> MALMTWTAAEFGT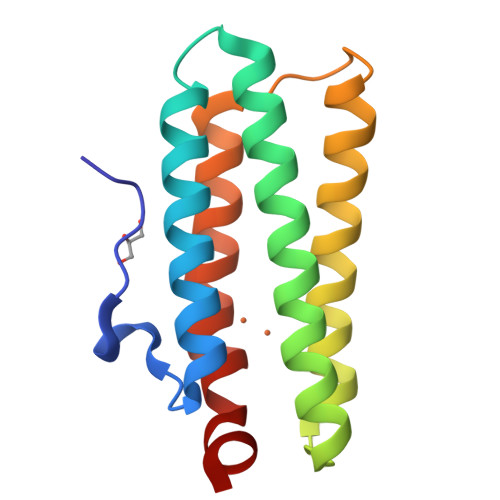NVGFADDQHKTIFDMVNKLHDTAATGNRSEIGKQLDALIDYVVMHFKSEETEMQKKGYADFAAHKAEHDKLVGVCADLQKKFHAGEAEVNQDTTRFVRDWFVNHIPKVDKLYGPCLSA>[4x]EPVQVFTDDLGRKVTVPAHPKRIVSLHDLDITIPLIELGVPPVASHGRTRPDGSHFIRSGALLTGVDFDNSSIAFIGTADIDIEAIVAAKPDLIITEPTRNTPIERLEKIAPTVSIDHLKGGAPEIYRKLAELTGTQSQLAILERRYQAQINALKATLDSQKITVSVIQANQGKINVMHSYHSLGRVLRDAGFRFPPLIESIPEGGRMDV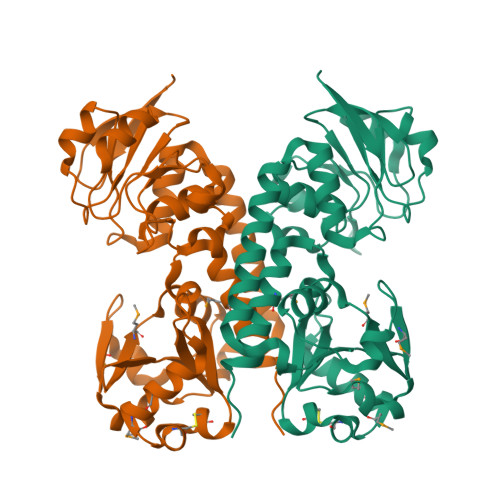SAERLPELDADFVFATWRGDTGGKPQDELATMEKVMPGWCQFLTACRSGRYVLISREEAISNSFASLGLMAAQIQSQIAGRPLPEAK> MLNPIVRKFQYGQHTVTLETGMMARQATAAVMVSMDDTAVFVTVVGQKKAKPGQDFFPLTVNYQERTYAAGRIPGSFFRREGRPSEGETLIARLIDRPIRPLFPEGFVNEVQVIATVVSVNPQVNPDIVAMIGASAALSLSGIPFNGPIGAARVGYINDQYVLNPTQDELKESKLDLVVAGTEAAVL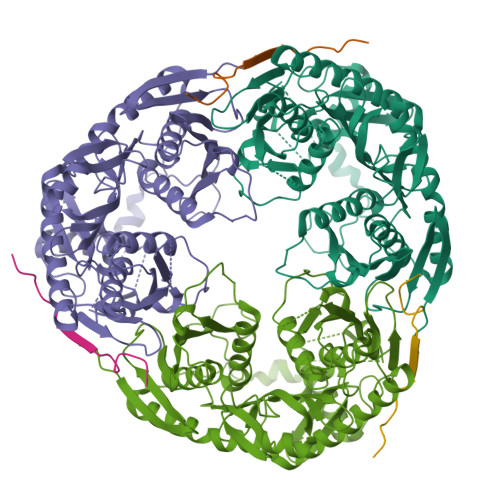MVESEAELLSEDQMLGAVVFGHEQQQVVIQNINELVKEAGKPRWDWQPEPVNEALNARVAALAEARLSDAYRITDKQERYAQVDVIKSETIATLLAEDETLDENELGEILHAIEKNVVRSRVLAGEPRIDGREKDMIRGLDVRTGVLPRTHGSALFTRGETQALVTATLGTARDAQVLDELMGERTDTFLFHYNFPPYSVGETGMVGSPKRREIGHGRLAKRGVLAVMPDMDKFPYTVRVVSEITESNGSSSMASVCGASLALMDAGVPIKAAVAGIAMGLVKEGDNYVVLSDILGDEDHLGDMDFKVAGSRDGISALQMDIKIEGITKEIMQVALNQAKGARLHILGVMEQAINAPRGDIS;> EAPRHSDWQRPTFAFEGKGAAGGHTATHHASAAPARPQPVE~{N}-[3-[[4-[(4-bromophenyl)methyl]piperazin-1-yl]methyl]phenyl]-2-ethyl-2-methanoyl-butanamide 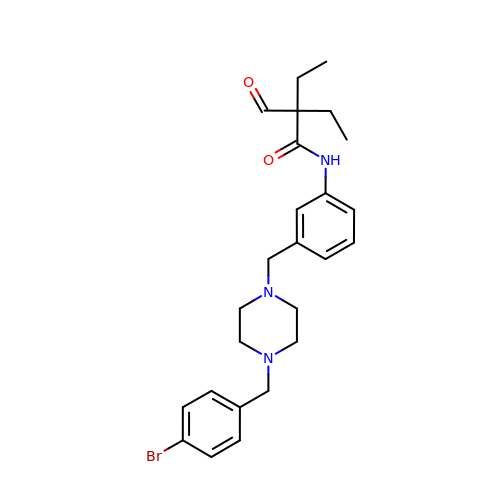| C25 H32 Br N3 O2 | LULPAFAMHVUJQY-UHFFFAOYSA-N> MTRHKTFRLVVDALLMAIVLLQNLVPFLGYIPFGPFSMTLIGLTVIVAGSALGP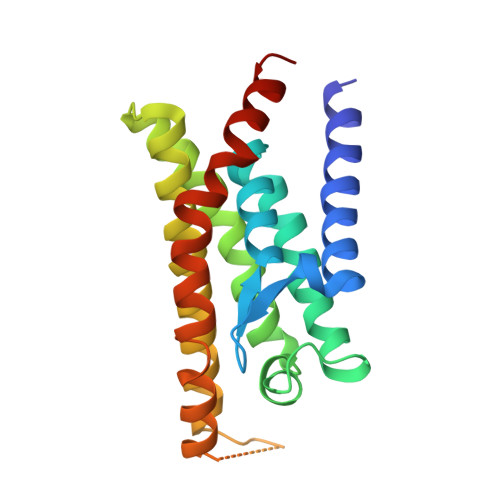RDGLLIGGFWGLITFVRAFTWPSSPVAPLIFTNPLISILPRLLMGLVAGSLYLWGRHRQWSMRQAMQVAAGCAALTNTVLVLGLVFLFYQTPAVATAFGATGNQTLGYVLMISLFTNGIPELILDVLVAPLIAMPLRRQWERLKPQTTK>[2x]GSGNSHTTPWTNPGLAENFMNSFMQGLSSMPGFTASQLDNMSTIAQSMVQSIQSLAAQGRTSPNKLQALNMAFASSMAEIAASEEGGGSLSTKTSSIASAMSNAFLQTTGVVNQPFI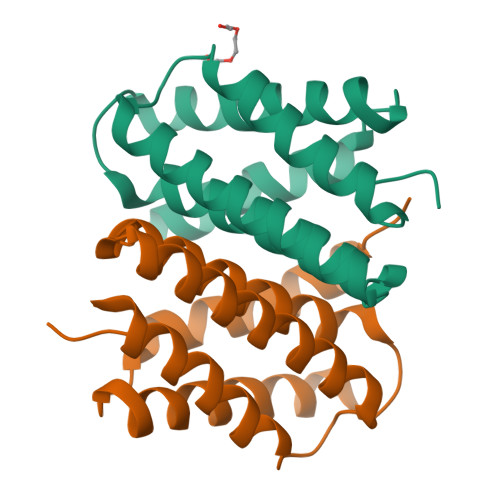NEITQLVSMFAQAGMNDVSA>SKVKGSQGQFPLTQNVTVVEGGTAILTCRVDQNDNTSLQWSNPAQQTLYFDDKKALRDNRIELVRASWHELSISVSDVSLSDEGQYTCSLFTMPV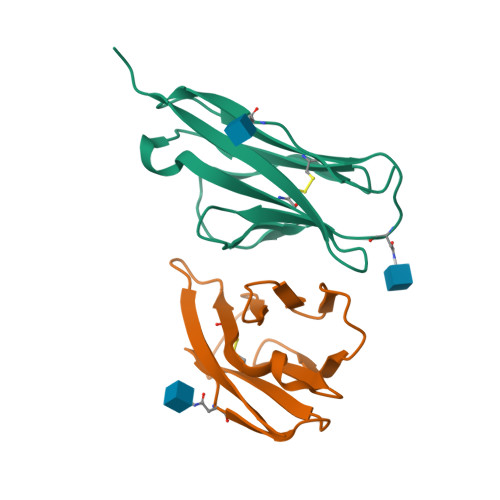KTSKAYLTVLGVP[4x]>GAMKSQEYTLIKIFVSNVKDFYSIFMNSIRSSQSVLNACIEKKEAPNNNNNKINNNKINGTFFTDFEKGEEDLKNKIWNEDFFVKDKKVIFLGSTLKPETAYGQNYTFINPNEYYYLTLGFDKQNLHYGDKSYVNNIMTKEEIINSCPNIYVCSENSLYNLAYQGIIPLLKNKNGNLDDVFILNKIKGEHFVGLETYTNISKIKNLYILPMTTIKMNISTGIVPCVSSDSTDDYACLEDIRKKKNYYCEKYNLKEEQLKNNSESCIELPEIGNNTGKYYYEKEKVSSYKDVKLQKIKEVLYK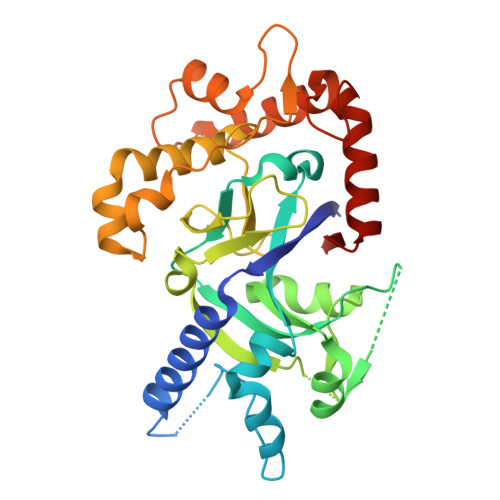KQYFEGIMTVDPYKGMKTFNCRKLAKQNIIRNLDGFLYSE[2x]>GAARIMLLERTLQLKEEENKRLNQRLMSQSMSSVSSRHSEKIAIRDFQVGDLVLIILDERHDNYVLFTVSPTLYFLHSESLPALDLKPGEGASGASRRPWVLGKVMEKEYCQAKKAQNRFKVPLGTKFYRVKAVSWNKKV[6x]

The formation of autophagosomes requires the hierarchical action of a number of conserved factors, including the upstream-acting ULK1 complex containing the scaffold protein FIP200 and the downstream-acting conjugation machinery, which catalyzes the conjugation of the ubiquitin-like ATG8 proteins to the head group of phosphatidylethanolamine on the isolation membrane. Crystal structure determination shows that the FIP200 CTR contains a dimeric globular domain that we designated the “Claw” for its shape. The interaction of p62 with FIP200 is mediated by a positively charged pocket in the Claw, enhanced by p62 phosphorylation, mutually exclusive with the binding of p62 to LC3B, and it promotes degradation of ubiquitinated cargo by autophagy. The Claw is constituted of a six stranded, mostly antiparallel β sheet and a short α-helix.

To gain mechanistic insights into the FIP200-p62 interaction, we determined the X-ray structure of the FIP200 CTR (aa 1458–1594). Crystals of this construct diffracted to a resolution of 3.2 Å and the phase problem was solved by a single anomalous dispersion approach using selenomethione-substituted crystals. A monomer of the FIP200 CTR comprises an N-terminal extended helix of 29 amino acids and a C-terminal globular domain of 100 amino acids to which we refer as the “Claw”. The connecting linker between the helix and the Claw is resolved in two out of six monomers. Accordingly, the Claw shows some flexibility relative to the helix. The six monomeric Claws in the asymmetric unit superimpose almost perfectly, with a root mean square deviation (rmsd) of their Cα atoms of 0.33 Å. Homodimerization of FIP200 CTR is mediated by the Claw (interface-1) and the N-terminal helices that form a coiled-coil (interface-2). The linkers cross each other in such a way that the Claw of one monomer sits on top of the coiled-coil helix of the second monomer. Dimerization buries an extensive surface area of 1,440 Å2, suggesting a physiologically plausible assembly. Along with these results, analytical size exclusion chromatography coupled to right-angle light scattering confirmed the dimeric nature of FIP200 CTR.> FDCAEYRSTNIYGYGLYEVSMKPAKNTGIVSSFFTYTGPAHGTQWDEIDIEFLGKDTTKVQFNYYTNGVGGHEKVISLGFDASKGFHTYAFDWQPGYIKWYVDGVLKHTATANIPSTPGKIMMNLWNGTGVDDWLGSYNGANPLYAEY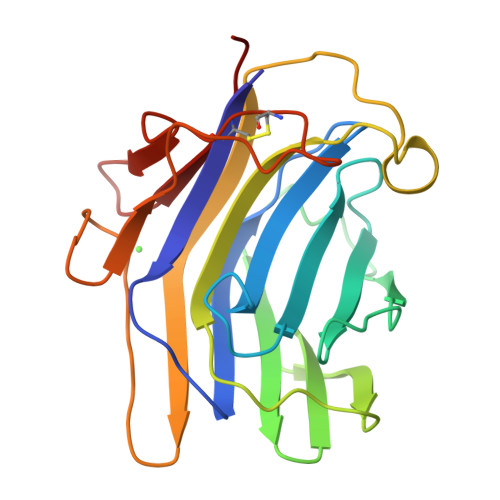DWVKYTSNGSVFWEPKSYFNPSTWEKADGYSNGGVFNCTWRANNVNFTNDGKLKLGLTSS> MVNKYTYTSSKAMSDISDVIGEPLAAWDSQVGGRVFNVIFDGKVYTNTYWVERWQVPGIGSSDGNPHNAWKFVRAATADEINKIGNPTTADVKPTENIPSPILVEDKYTEETYSRPDVNFKEDGSQGNLSYTATRVCAPMYNHYVGDKTKPKLSAYITDWCQYDARLDGGGSKEEERGRGFDLATLMQNPATYDRLIFSFLGICGDIGNKSKKVQEVWDGWNAQAPSLGLPQIGKGHIVPLDPYGDLGTARNVGLPPESADTSIESGTFLPYYQQNRAAGLLGGLRELQKKAHAMGHKLDLAFSIGGWSLSSYFSALAENPDERRVFVASVVDFFVRFPMFSCVDIDWEYPGGGGDEGNISSDKDGENYVLLIKELRSALDSRFGYSNRKEISIACSGVKAKLKKSNIDQLVANGLDNIYLMSYDFFGTIWADYIGHHTNLYSPKDPGEQELFDLSAEAAIDYLHNELGIPMEKIHLGYANYGRSAVGGDLTTRQYTKNGPALGTMENGAPEFFDIV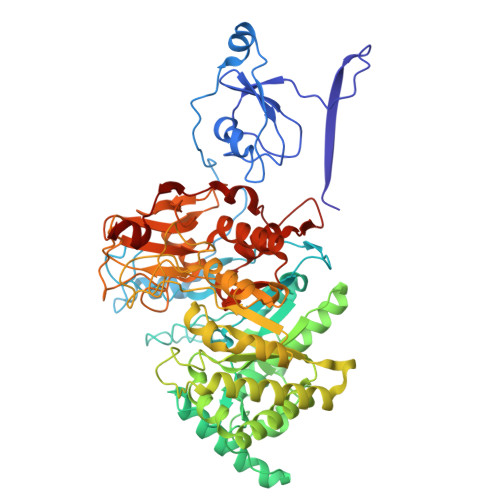KNYMDAEHSLSMGKNGFVLMTDTNADADFLFSEAKGHFISLDTPRTVKQKGEYAAKNKLGGVFSWSGDQDCGLLANAAREGLGYVADSNQETIDMGPLYNPGKEIYLKSISEIKSK(6S,9aS)-6-[(2S)-butan-2-yl]-8-[(1R)-1-naphthalen-1-ylethyl]-4,7-bis(oxidanylidene)-N-[4,4,4-tris(fluoranyl)butyl]-3,6,9,9a-tetrahydro-2H-pyrazino[1,2-a]pyrimidine-1-carboxamide | C28 H35 F3 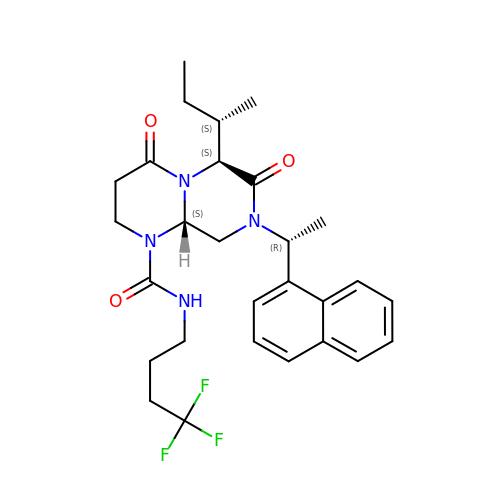N4 O3 | BAZGDIOJCKGDHH-RHDWJPPYSA-N> GIDELYKKEFGIVAGVDEASRGCLAGPVVAAAVVLEKEIEGINDSKQLSPAKRERLLDEIMEKAAVGIGIASPEEIDLYNIFNATKLAMNRALENLSVKPSFVLVDGKGIELSVPGTCLVKGDQKSKLI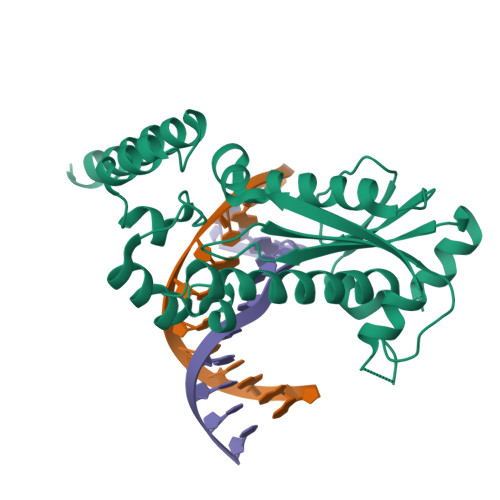GAASIVAKVFRDRLMSEFHRMYPQFSFHKHKGYATKEHLNEIRKNGVLPIHRLSFEPVLELLTDDLLREFFEKGLISENRFERILNLLGARKSVVFRKERTNHNLPLF> MVSELIKENMPMKLYMEGTVNNHHFKCTSEGEGKPYEGTQTMRIKVVEGGPLPFAFDILATSFMXGSRTFIKHPPGIPDFFK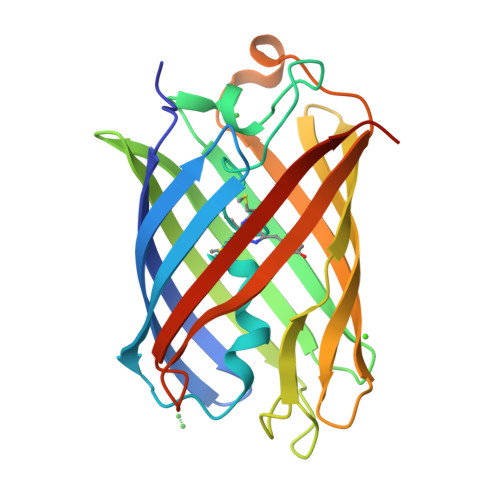QSFPEGFTWERVTTYEDGGVLTATQDTSLQDGCLIYNVKVRGVNFPANGPVMQKKTLGWEASTETMYPADGGLEGACDMALKLVGGGHLICNLETTYRSKKPATNLKMPGVYNVDHRLERIKEADDETYVEQHEVAVARYSTGGAGDGGK>[3x]M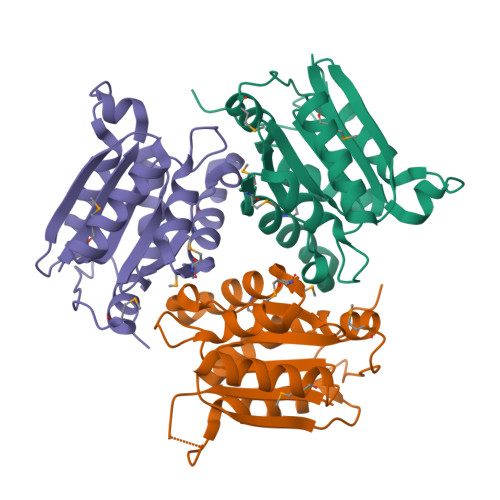SKAKIGIVTVSDRASAGIYEDISGKAIIDTLNDYLTSEWEPIYQVIPDEQDVIETTLIKMADEQDCCLIVTTGGTGPAKRDVTPEATEAVCDRMMPGFGELMRAESLKFVPTAILSRQTAGLRGDSLIVNLPGKPKSIRECLDAVFPAIPYCIDLMEGPYLECNEAVIKPFRPKAK> QVASEYLGGPGGDAFDDKALAQNGDITRIEMQCTDVATYIKLRYGKVDSRQWGWANENCIQWSKKGVKVVHELSSGEYITSAIVTYGKYVQSITFKTNKRTLPRCGTSATEKSVTVLIPGGLKYISGRWGCRIDGLRFH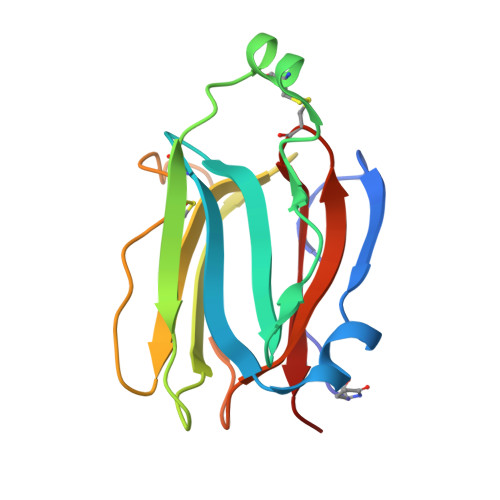AKC> EASIPTVERSTRMSNPWKAFME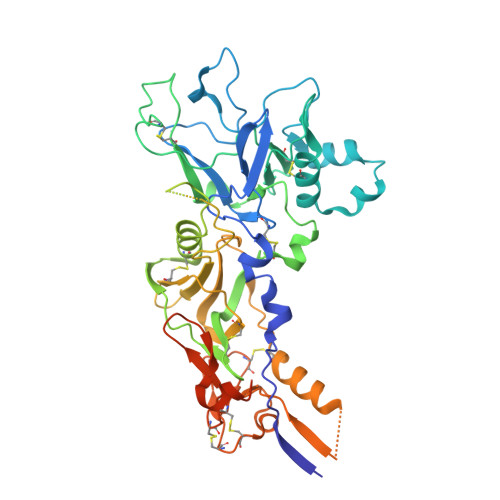KYDIERTHSSGVRVDLGEDAEVENAKYRIPAGRCPVFGKGIVIENSDVSFLRPVATGDEKLKDGGFAFPNANDHISPMTLANLKERYKDNVEMMKLNDIALCRTHAASFVMAGDQNSNYRHPAVYDEKEKTCHMLYLSAQENMGPRYCSPDAQNRDAVFCFKPDKDESFENLVYLSKNVRNDWDKKCPRKNLGNAKFGLWVDGNCEEIPYVKEVEAEDLRECNRIVFGASASDQPTQYEEEMTDYQKIQQGFRQNNREMIKSAFLPVGAFNSDNFKSKGRGFNWANFDSVKKKCYIFNTKPTCLINDKNFIATTALSHPQEVDLEFPCSIYKDEIEREIKKQSRNMNLYSVDGERIVLPRIFISNDKESIKCPCEPERISQSTCNFYVCNCVEKRAEIKENNQVVIKEEFRDYYENGEEKSNKQMLLLEQKLISEEDLNSAVDHHHHHH N-(trifluoroacetyl)-L-phenylalanyl-N-[4-(trifluoromethyl)phenyl]-L-alaninamide | C21 H19 F6 N3 O3 | 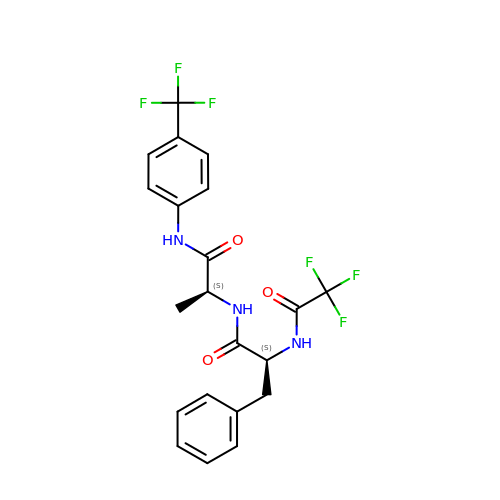YVHDCJDFGBMJNF-LRDDRELGSA-N>MWSHPQFEKGGSGNSGQNLENIKKFIRAANYLTVSQIFLQDNFLLERPLTFEDIKPRLLGHWGSCPGVNWVYAHLLNIQKQLEFAKSGLKAAFMLGPGHAFPALQANLFMEETLSKVDKKATRNAQGIEYISKNFSWPGGFPSSASPFTPGVILEGGELGYSLSTAFGAILDNPNLVMTTLIGDGEAETGSIAAAWHLSKLIDPVKNGVVLPVLHLNGYKISGPTIFGSMSDFELIQFFHGAGWEPKIVDEYSAEDFDLELSNAFSNAFRDISRIKFGRNSKFIRLPMIIMRSKKGSSGVKENNGQKIEGNSLAHQVPLLKAKTDKNELEKLENWMKSYKFDELFDYERGEFKWWINDFLPENSSRIGRNRFVDANLNFKELKLPEITEGFGEKSLAMNAVGSLLEKVFEKNPDNFRFFSPDETYSNKLDAIFEATSRSWQREIKPWEKDLAKNGRVTEILSENCLQGLLQGYILTGRYGVLTSYEAFAPVISSMMDQYAKFLAQSKEVKWRGDLASLNYILTSTGWRQDHNGFNHQNPSFIDEVLRRENGIGQIFLPADDNSAVAAISKMLKTRNNINVLVAGKTPEPRYFSL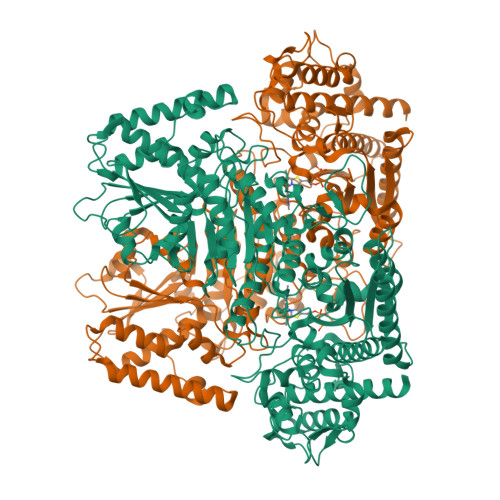ESAQKQLENGGIFVFDSWKNQKITDWDSISEDDEPDLILAASGDYVFKETVAALQVLLHDVAQVKIRLVYIQALCGKGIGTFENTLSKSDFVKIFTKDKPVIFAFHGYAKTLKSILFDYENPARIQINGYEEKGSTTTPFDMLARNKVSRYDITVRALKSVSEGDKVFGSLVKEYRKRQDDALRFAQENSVDAPEIENWDYLRFF[2x]>PKISLQIPIKLKSVLVDDWEYVTKDKKICRLPADVTVEMVLNKYEHEVSQELESPGSQSQLSEYCAGLKLYFDKCLGNMLLYRLERLQYDELLKKSSKDQKPLVPIRIYGAIHLLRLISVLPELISSTTMDLQSCQLLIKQTEDFLVWLLMHVDEYFNDKDPNRSDDALYVNTSS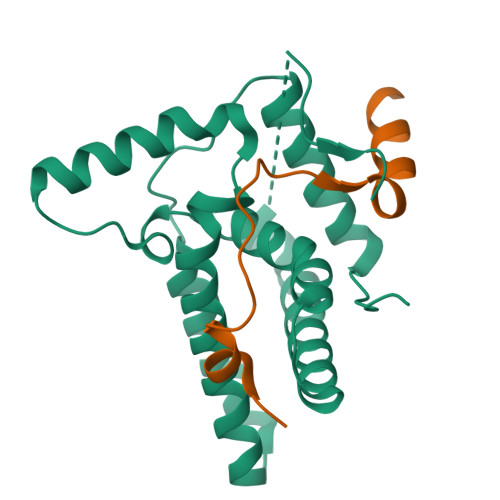QYEGVALGM[2x];>EETLLELNNRIRVRKQDFTLPWEEYGELILENARKS[2x]> GSH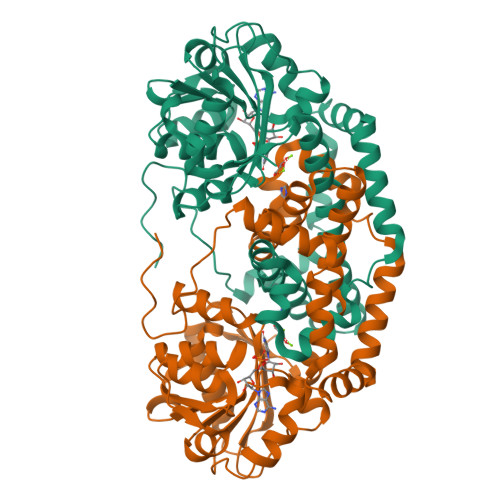MASNDLIYQDEHASLQPLEGRTVAVIGYGIQGRAFAANLRDSGVAVRVGNIDDRYFELARAEGHRVTNIAEAVAHADIVLLLIPDEAHGAVFDVDIAPNLRDGALLCVAHGHSLVQGDVRPLPGRDLAMLAPRMYGDPIRRYYLAGQGAPAYFDIVADHTGRARDRVLAIARAVGFTRAGVMALGYRQETFLDLFQEQFLAPALVDLVETGFQVLVERGFNPKAALLEVYGSGEMGKMMLDGADIGLDEVVALQGSPTCQVGYHRWRGRTLPTAVRELAARVLDQIEGGDFSAYLKEQASNDYASLDDARRAALKRPLNVAHAQVRAAFRFPTEAAGGLYQAAQAPADVEPEAAR> QEERNQQQDDIEELETKAVGMSNDGRFLKFDIEIGRGSFKTVYKGLDTETTVEVAWCELQDRKLTKSERQRFKEEAEMLKGLQHPNIVRFYDSWESTVKGKKCIVLVTELMTSGTLKTYLKRFKVMKIKVLRSWCRQILKGLQFLHTRTPPIIHRDLKCDNIFITGPTGSVKIGDLGLATLKRASFAKAVIGTPEFMAPEMYEEKYDESVDVYAFGMCMLEMATSEYPYSECQNAAQIYRRVTSGVKPASFDKVA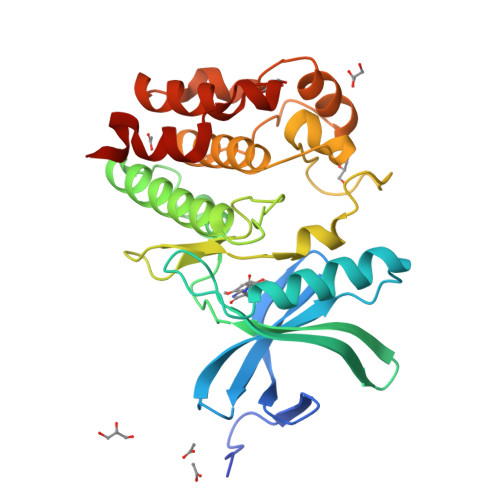IPEVKEIIEGCIRQNKDERYSIKDLLNHAFFQEET> EVVKLLLEHGA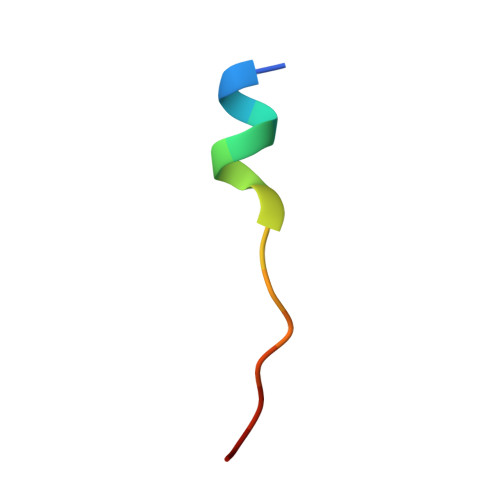DVXA>FACKTANGTAIPIGGGSANVYVNLAPVVNVGQNLVVDLSTQIFCHNDYPETITDYVTLQRGSAYGGVLSNFSGTVKYSGSSYPFPTTSETPRVVYNSRTDKPWPVALYLTPVSSAGGVAIKAGSLIAVLILRQ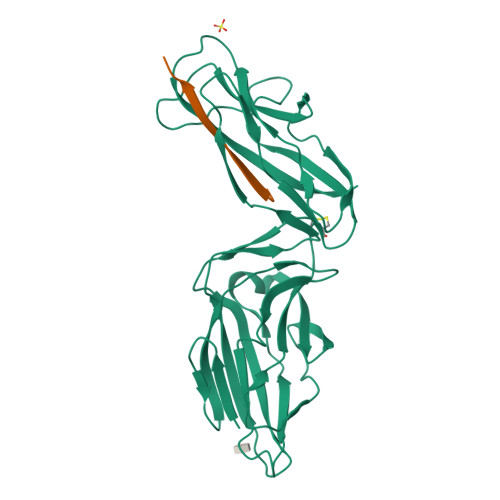TNNYNSDDFQFVWNIYANNDVVVPTGGCDVSARDVTVTLPDYPGSVPIPLTVYCAKSQNLGYYLSGTTADAGNSIFTNTASFSPAQGVGVQLTRNGTIIPANNTVSLGAVGTSAVSLGLTANYARTGGQVTAGNVQSIIGVTFVYQ[4x];>ADSTITIRGYVRDNG[4x]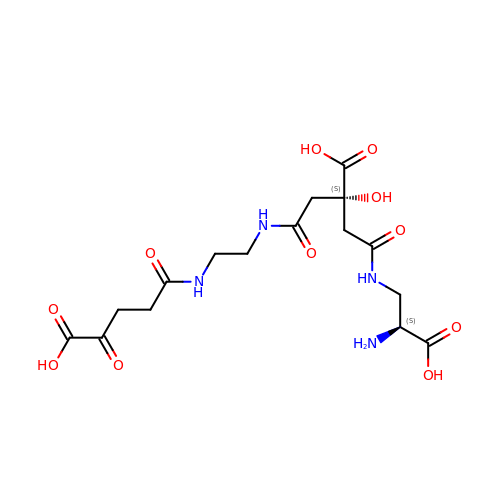5-[(2-{[(3S)-5-{[(2S)-2-amino-2-carboxyethyl]amino}-3-carboxy-3-hydroxy-5-oxopentanoyl]amino}ethyl)amino]-2,5-dioxopentanoic acid | C16 H24 N4 O11 | SIAZVTIHOHTZDD-PWJLMRLQSA-N> G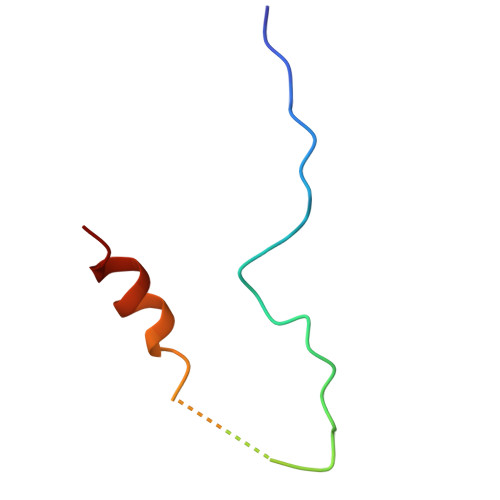MSQVKSSYSYDAPSDFINFSSLDDEGDTQNIDSWFEEKANLEN> KETAAAKFER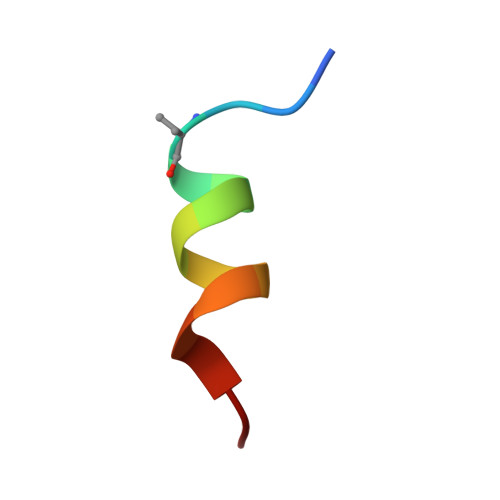QHLDS> MCPQKLTISWFAIVLLVSPLMAMWELEKDVYVVEVDWTPDAPGETVNLTCDTPEEDDITWTSDQRHGVIGSGKTLTITVKEFLDAGQYTCHKGGETLSHSHLLLHKKENGIWSTEILKNFKNKTFLKCEAPNYSGRFTCSWLVQRNMDLKFNIKSSSSSPDSRAVTCGMASLSAEKVTLDQRDYEKYSVSCQEDVTCPTAEETLPIELALEARQQNKYENYSTSFFIRDIIKPDPPKNLQMKPLKNSQVEVSWEYPDSWSTPHSYFSLKFFVRIQRKKEKMKETEEGCNQKGAFLVEKTSTEVQCKGGNVCVQAQDRYY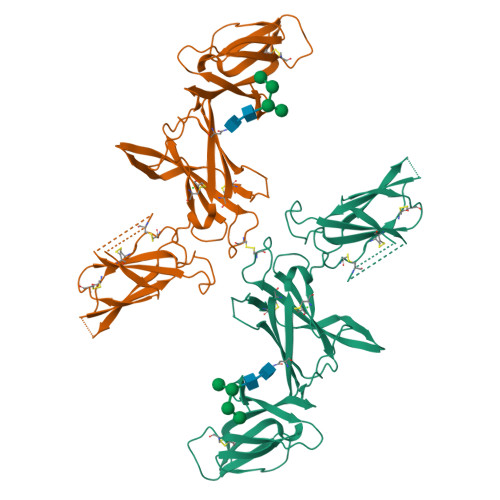NSSCSKWACVPCRVRSGTKHHHHHH Retromer is a master regulator of cargo retrieval from endosomes, which is critical for many cellular processes including signaling, immunity, neuroprotection, and virus infection. The core of retromer is a trimer comprising vacuolar protein sorting (VPS) proteins VPS35, VPS26, and VPS29. Here, we elucidate the structural basis of membrane tubulation and coupled cargo recognition by metazoan and fungal retromer coats assembled with the non–Bin1/Amphiphysin/Rvs (BAR) sorting nexin SNX3 using cryo–electron tomography. The retromer core retains its arched, scaffolding structure but changes its mode of membrane recruitment when assembled with different SNX adaptors, allowing cargo recognition at subunit interfaces.

Cryo–electron tomography revealed the architecture of fungal retromer core assembled on membranes via a membrane adaptor, a dimer of sorting nexins (SNX) containing Bin1/Amphiphysin/Rvs (BAR) domains, in which the core trimer forms an arch-like structure over a layer of SNX-BAR adaptors. BAR domains are known for their curvature-generating/stabilizing properties, and the accepted dogma is that membrane curvature enabling the formation of tubules is induced by the SNX-BARs, with retromer core trimer playing an auxiliary role. In the assembled retromer:SNX-BAR, the core trimer does not contact the membrane but is bound to the SNX-BAR adaptor layer via loops 5 and 9 of VPS26 (6). In retromer:PX-BAR coats, membrane bending will be enhanced through the well-established local membrane-remodeling action of the curved BAR domains. The core trimer arch—the conserved architectural element of the different retromer coats—forms a scaffold that can contribute directly or indirectly to membrane bending and which propagates curvature over larger areas of membrane by oligomerization.

>MSTPAPPEEQARLLEDALIAVRQQTAMMRKFLDTPGKLMDALKCCSTLVSELRTSSLSPKQYYELYMAVFDALRYLSAHLRENHPVNHLADLYELVQYAGNIIPRLYLMITVGTAYMSIDGAPVKELMKDMMDMSRGVQHPVRGLFLRYYLSGQARDYLPTGDSDGPEGNLQDSINFILTNFVEMNKLWVRLQHQGHSRERDLRTQERRELQLLVGSNIVRLSQLVDLPTYRDSILGPLLEQIVQCRDILAQEYLLEVITQVFPDEYHLHTLDQFLGAVSRLNPHVNVKAIVIGMMNRLSDYAERESQNEPEEDRAKLEEEALAKLLEKTKLGQNSELEPQNGDHPDTEVSSTTDSAQAPSTADSDTTAVNGEEEPVRKRRGIPVNVPLYDIFFDQVQHLVQAQHLPIQDTIALCCSLANLSLNIYPERLDYVDGILAYALAKVKEHANSADLHSQPAQQSLLSLLQSPLRRYVSIFTALSLPTYVSLFQAQTYPTRRAIAGEIVRTLLKNQTLISTPAHLENVLEILKVLIKEGSQPPAGYPGVVQPRARPLETDETMEEQGWLARLVHLIHSDDNDTQFRLLQMTRKAYAEGNERIRTTTPPLITAGLKLARRFKAREHYDDNWSSQSSSLFKFLHSAISTLYTRVNGPGVADLCLRLFCSCGQVADMTEFEEVAYEFFAQAFTVYEESISDSKAQFQAVCVIASALHRTRNFGRENYDTLITKCAQHASKLLRKPDQCRAVYLASHLWWATPIAARGETEDTELYRDGKRVLECLQRALRVADSCMETATSIELFVEILDRYVYYFDQRNESVTTKYLNGLIELIHSNLAGNQQDSASVEASRKHFIQTLEMIQSKEFEGIVVAPK[2x];>SMAFLILVIGNLHIPDRALDIPPKFKKLLSPGKISQTLCLGNLTDRATYDYLRSISPDLKIVRGRMDVEATSLPLMQVVTHGSLRIGFLEGFTLVSEEPDVLLAEANKLDVDVLCWAGGSHRFECFEYMDKFFVNPGSATGAFTTDWLAEGEEVVPSFCLMDVQGISLTLYVYQLRKDENGTENVAVEKVTYTKPVEPTGAS[2x]>GTSSMADIGSRYSKISDNYSSLLQVSEALGRAGLESSNLIVGIDFTKSNEWTGAKSFNRKSLHHLSNTPNPYEQAITIIGRTLAAFDEGNLIPCYGFGDASTHDQDVFSFYPEGRFCNGFEEVLARYREIVPQLKLAGPTSFAPIIEMAMTVVEQSSGQYHVLVIIADGQVTRSVDTEHGRLSPQEQKTVDAIVKASTLPLSIVLVGVGDGPWDMMQEFDDNIPARAFDNFQFVNFTEIMSKNKDQSRKETEFALSALMEIPPQY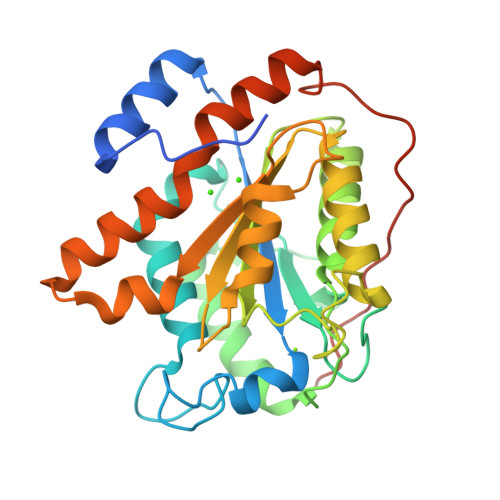KATIELNLLGVRNGNIPQRIPLPPPVQSGSSFSSSR[8x]>[3x]GPAVPRMVVLHSLLGMAVLIAIAVL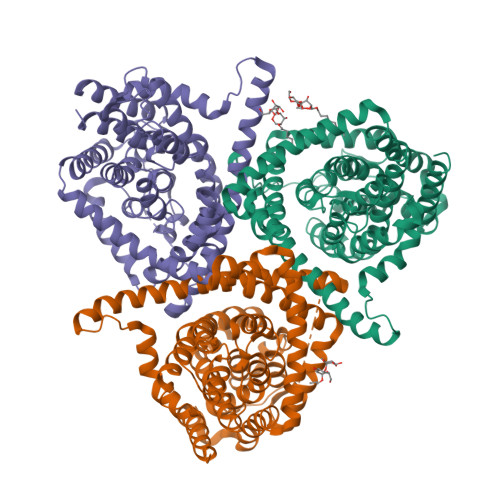LSTDRKAINIRTVAGAFLIQVALGALVLYVPQGRDMLGEASKTISNVIAYGNNGVDFLFGGLVSEKMFEVFGGGGFVFALRVLPMIVFFSSLMAVLYYIGVMQLLIKVIGGFLQKMLGTSKAESMSAAASIFVGQTEAPLVVRPYIRRMTESELFAVMSGGLASVAGSVLAGYVQMGVPLPYLIAASFMAAPGGLLFAKLLVPETERTQNDAEVLAENEDEKPTNVIDAAASGAVTGAQIAIAVGASLLAFVALIAMINGIIGGVGGWFGHGDLTLQAILGWLFSPLAWVIGVPWSEAGIAGSLIGQKVVINAFVAYSEFVKYLKPEAAVQLSDTTKAIISFALCGFANLGSIAVLVGGLSIMAPKRRKDVARLGIKAVVAGSLSNLMSAVIAGLFTGLSGASVLG The Scribble (Scrib) protein is a conserved cell polarity regulator with anti-tumorigenic properties. Scribble is an important regulator of cell polarity and acts as a scaffolding protein to mediate a diverse set of cellular signalling pathways via its four PDZ domains. The zoonotic Tick-born encephalitis virus TBEV encodes for the NS5 protein, which has been shown to interact with Scribble in a PDZ domain dependent manner. In summary, we show that TBEV NS5 C-terminal PBM binds SCRIB PDZ3 in order to interact with Scribble.

To understand the interactions of SCRIB PDZ domain interactions with NS5 PBM sequences in more detail we determined crystal structures of SCRIB PDZ3:NS5_CTN complexes as well as a structure of SCRIB PDZ3 apo. Isothermal titration calorimetry revealed that only the C-terminal PBM NS5_CTN bound to SCRIB PDZ3 with a KD value of 18.4 ± 1.3 µM. In the Scrib PDZ3:NS5_CTN complex, His1071PDZ3 contacts Ser3412NS5 in the −2 position in the canonical manner observed in many other PDZ domain complex structures. Our crystal structure of SCRIB PDZ3 bound to PBM sequences revealed an interaction with a conserved His residue. Mutation of SCRIB PDZ3 H1071 to Ala ablates binding, whereas mutation of SCRIB PDZ3 K1040, which is not involved in NS5 engagement, did not significantly impact binding affinity. This supports the notion that SCRIB PDZ3 H1071 plays an important role in the NS5 CTN engagement.

>GPLGSSAPSVKGVSFDQANNLLIEPARIEEEELTLTILRQTGGLGISIAGGKGSTPYKGDDEGIFISRVSEEGPAARAGVRVGDKLLEVNGVALQGAEHHEAVEALRGAGTAVQMRVWRERM[2x];>EMYYSTAV[2x]> GAGC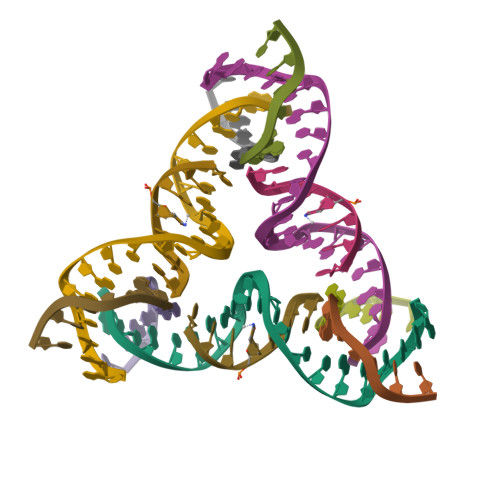AGCCTGTTTGGACATCA;> CCACACA;> GGCTGCT;> CTGATGT>[2x]GPSYHCKTPDCKGWCFFEDDVNEFTCPVCFHVNCLLCKAIHEQMNCKEYQEDLALRAQNDVAARQTTEMLKVMLQQGEAMRCPQCQIVVQKKDGCDWIRCTVCHTEICWVTKGPRWGPGGPGDTSGGCRCRVNGIPCHPSCQNCH

LUBAC is a heterotrimeric ligase which consists of the three proteins HOIP, HOIL-1 (also known as RBCK1) and SHARPIN. Two of the LUBAC components display Ub ligase activity, HOIP and HOIL-1, and both belong to the family of RBR (Ring-between-RING) ligases. HOIL-1 is a member of the RBR E3 ligase family with the ability to ubiquitylate its targets by linking a hydroxy group of the substrate to the C-terminus of Ub. We show that HOIL-1 activity requires linear tetra-Ub binding which enables HOIL-1 to mono-ubiquitylate linear Ub chains and polysaccharides.

To elucidate the structural features which enable HOIL-1 to exert its unique catalytic activity we solved the crystal structure of fragment 366–510, which comprises the IBR and the RING2 domain. The overall structure shows that both domains are linked by two helices, which are positioned at a 50 angle. This arrangement brings the IBR and the RING2 domains into close vicinity to each other and allows them to form an interface which buries a total of 1,303 A2 of solvent accessible surface area. K457 of RING2 is a central contact point for the IBR domain, and is coordinated by F382, E383, V386, and N387. The C-terminal histidine (H510) of RING2 forms a polar interaction with D385 of the IBR domain. These interactions, together with further hydrophobic and polar contributions by D458, K456, Q455, I452, V467, and R464 in RING2 with N387, K403, and L401 of the IBR, create a surface which largely obstructs the catalytic cysteine C460. We therefore assume that the observed structural arrangement represents a catalytic inactive conformation of HOIL-1 in which the catalytic cysteine of RING2 is masked by the IBR domain. As expected from our sequence analysis, the C-terminal part of the RING2 domain of HOIL-1L reveals a unique architecture not observed in other RBR ligases so far: The C-terminal 36 residues form a loop structure which is laced up by a binuclear Zn cluster coordinated by six cysteines. This structure adopts a compact conformation which packs against the second beta sheet of the canonical RING2 fold. HOIL-1 displays a tryptophan (W462) instead of a histidine located two amino acids downstream of the catalytic cysteine, questioning if HOIL-1 requires a histidine to assist catalysis as observed for other RBR ligases. The C-terminal residue of HOIL-1 is a histidine (H510) which forms a pi-staking interaction with W462.> GAGCAGACCCGA;> CGGGACTCA;> TCGCCG;> TCTGAGTCGGTCTGC

In this work, we exhaustively probe the ability of all 36 immobile HJ sequences to form DNA crystals in two different designed systems. Three separate self-assembling DNA crystal systems are described in this report: the “4 × 5” and “4 × 6” designs (collectively referred to as the 4 × N systems), and a third construct with a “scrambled” sequence variant of the 4 × 6 lattices. Self-assembly was mediated by three constituent oligonucleotides: (S1) containing four sequence repeats of either 5 or 6 bases; (S2) composed of 21 bases containing complementary regions to both (S1); and (S3) which forms the second junction crossover. The HJ serves as the fundamental component at the core of each unit, and the ultimate assembly of the full lattice is facilitated by the complementary 2-base sticky ends that tail each duplex.

In parallel, we employed the previously reported J1 4 × 6 system (3.05 Å), with P32 symmetry. Seventeen of the 36 junctions successfully crystallized, a 47% success rate. Unlike the 4 × 5 motif, nearly all of the 4 × 6 junction sequences had a strong preference for crystallization in buffers containing ≥2.0 M salts (e.g., LiCl, Li2SO4, KCl, and NaCl), with the majority preferring slightly basic pH conditions in cacodylic acid. The average cell constants for the P32 crystals were a = b = 68.29 Å c = 55.68 Å. The c-axis, in particular, was ~5 Å shorter, and had a much larger degree of variability (σ = 1.97), than those that crystallized using the 4 × 5 motif. The broad range of the short axis spanned from 52.77 to 60.36 Å, and we posit that the flexible axis lengths could be responsible for rendering a larger number of junctions fatal than the 4 × 5 system.>[2x]MTDLKASSLRALKLMDLSTLNGDYTDEKVIALCHQAKTPVGNTAAISVYPRSIPIARKTLKEQGTPEIRIATVTNFPHGNDDIEIALAETRAAIAYGADEVDVVFPYRALMAGNEQVGFDLVKACKEACAAANVLLKVIIETGELKDEALIRKASEISIKAGADFIKT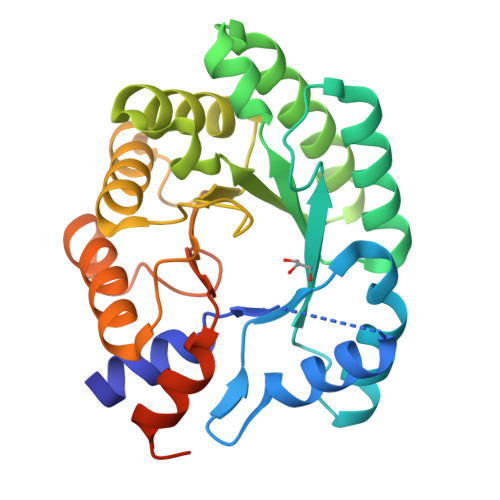STGRVAVNATPESARIMMEVIRDMGVEKSVGFKVTGGVSTAEDAQKYLAIADELFGADWADARHYRFSASGLLASLLKALGHGDGKSASSYLEHHHHHH>[14x]SGFASPAPANSETNTLPHVAFYISVNRAISDEECTFNNSWLWKNEKGSRPFCKDANISLIYRVNLERSLQYGIVGSATPDAKIVRISLDDDSTGAGIHLNDQLGYRQFGASYTTLDAYFREWSTDAIAQDYRFVFNASNNKAQILKTFPVDNINEKFERKEVSGFELGVTGGVEVSGDGPKAKLEARASYTQSRWLTYNTQDYRIERNAKNAQAVSFTWNRQQYATAESLLNRSTDALWVNTYPVDVNRISPLSYASFVPKMDVIYKASATETGSTDFIIDSSVNIRPIYNGAYKHYYVVGAHQSYHGFEDTPRRRITKSASFTVDWDHPVFTGGRPVNLQLASFNNRCIQVDAQGRLTANMCDSQQSAQSFIYDQLGRYVSASNTKLCLDGAALDALQPCNQNLTQRWEWRKGTDELTNVYSGESLGHDKQTGELGLYASSNDAVSLRTITAYTDVFNAQESSPILGYTQGKMNQQRVGQDNRLYVRAGAAIDALGSASDLLV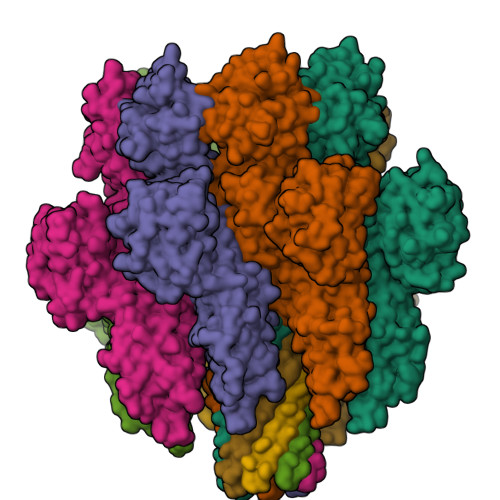GGNGGSLSSVDLSGVKSITATSGDFQYGGQQLVALTFTYQDGRQQTVGSKAYVTNAHEDRFDLPDAAKITQLKIWADDWLVKGVQFDLN>MAEDPDPTEYLYISMEQKRKDQTKPYDGKKMVWVADEKEGYLLGLIKSTQGDICTVDIEGQESRQVKKDLLQQVNPPKYEKCEDMSNLTYLNDASVLHNLKQRYYANLIYTYSGLFCVAINPYKRFPIYTNRTVQIYKGRRRTEVPPHLFAISDGAYSAMLANRENQSMLITGESGAGKTENTKKVIAYYANVGAATPKPGKEAPTKEKKATLEDQVVQTNPVLEAFGNAKTVRNDNSSRFGKFIRIHFGPMGKLAGADIETYLLEKARVISQQTLERSYHIFYQLMSGGIENLKADLLLSDDIYDYHFVSQGKIEIPGVDDAEELRLTDTAFDILGFSHEYKTDVYKITASCMHLGEMKFKQRPREEQAEADGTEEGERVAHLLGVNAADLYKNLVKPKIKVGNEMVTQGRNATQVSYSVGGLAKAMFDRTFKWLVKRLNETLDTKQKRQYFIGVLDIAGFEIFDYNGFEQLCINFTNEKLQQFFNHHMFVLEQEEYKREGIDWVFIDFGLDLAACIELIEKPMGILSILEEESMFPKATDKSFQDKLNANHLGKSPNFVKPKPPKPGQQEAHFSIAHYAGTVPYNITGWLEKNKDPVNDTVVDQFKKGSNKLVQEIFEDHPGLGAEEKGGGGKGGGGRKKGASFQTVSALYREQLNRLMASLHSTQPHFVRCIIPNELKQPGVIDSGLVMHQLTCNGVLEGIRICRKGFPNRMVYPDFKQRYTILAASAVPKGFVDAKKVTEAVLGAIQLDANDYRLGNTKVFFRAGVLGRLEEMRDDRLGKIVTWLQAWIRWYLSKKEFKKLQEQRVALLVIQRNLRKFLTLRNWLWYKLYIKVKPLLTMAKVEDELKALEEKLKKALESLEKEEKVRKDIEVQNVKLLQEKNDLFLQLESERSGAGDVEERLTKAISMKNDLEGQVQELQERLSREEDAHSNLSSVRKKLDGEISNLKKEIEDLQL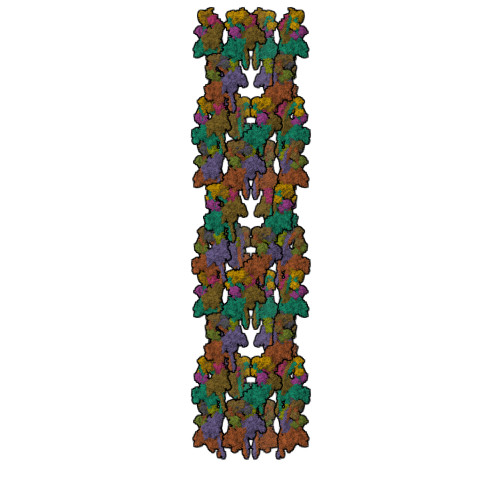VIQKTEQDKAAKDHQIRNLNDEIAHQDELINKLNREKKQMQEMGQKTGEDLQATEDKLNHMNKVKAKLEQTLDELEDSLEREKKLRGDVEKTKRKVEGDLKLAQEAVADLEKNKKELEQALQRKEKEMASLSAKLEDEQGLVAKLQKQIKELQARIEELEEELEAERQARAKAEKQRADLAREIEELSERLEEAGGATSAQVELNKRREAEMAKLRRDLEESNIQHEQTLANLRKKHNDVVAELSEQIDQLNKHKARLEKEKAQMKGELDDVRSSVDHVNKEKANAEKQAKQLEMQLTELQGKMDEAHRSLGDFDAAKKRLTVENTELTRQLEDAESQVSQLSKLKTSLQTQLEDTKRMADEESRERATAMGKFRSVEHDLDSLREQIDEEQEGKADLQRQLSKANAEVQLWRSKYESEGLARLEELEESKRKLDAKLQEAMETIDQLNSKTSGLEKTKSRLQGELEDMTIEVEKANALASAMEKKQKSFDRIISEWKQKVDDLALELDASQKECRNYSTEVFKLRSQYEESQEHYESVKRENKNLQDEIKDLVDQLGEGGRSVHELEKARKRLELEKEELQAALEEAEAALEQEENKVLRAQLELSQVRQEIDRRLQEKEEEFENTRKNHQRAIDSMQASLEAEAKGKAEALRMKKKLESDINELEIALDHSNKANAEAQKNIKKYQIQLKETQQALEEEQRARDEVREQYAMSERRCNAMHGELEESRQLLEQADRARRAADSELAELHENVNELSAQNSSLSMAKRKLEGEMQALHADLDEMLNEAKSSEEKAKKAMVDAARLADELRAEQEHAQQQEKMRKAMEGQIKELQVRLDEAEAAALKGGKKIIQKLEQKVRELETELDNEQRRHSEAAKNVRRSERRVKELQFQAEEDRKNQERMQDLVDKLQQKIKTYKRQIEEAEEIAALNLAKFRKVQQELEDAEERADMAENVAAKLRAKNRSSASVGRAMSPIPMGKPGRPKSKIDEE[4x];>MADLKAAEVEKAREHFEIYDWEGEGKIDARDLGDLLRSLDCKPTLAMVKKNGGSDKRGEKKLTLEEFLPIFSQIKKEKEVGTLEDFMEGLKVYDKAENGTMLAAELAHVLLSLGERLTDIECEEIMRVCDEDDDGFLKYEPFVKTIIAGPFPDEGK[4x];>[4x]MGDEEKKEKKKKSKKKSEEEGGDAAPAPPPPKPPSQKRRAQRSGSNVFAMFTQHQVQEFKEAFQLIDQDKDGFISKNDIRATFDSLGRLCTEQELDSMVAEAPGPINFTMFLTIFGDRIAGTDEEDVIVNAFNLFDEGEGKCKEETLKRSLTTWGEKFSQDEVEEALSEAPIDGNGLIDIKKFAQILTKGAEEEGA> MDHNTFWFILIAFLFSGYFLLEGFDFGVGILAPIIGKDSAARNTVIRTIGPVWDGNEVWLIVAGGALFAAFPEWYATMFSGMYLPLFLVLVSLIIRVVGLEWRKKVDDPRWQKWSDRAIFIGSWTPPLMWGFIFANILRGMPIKADHTIDAAAALPGMVNVFAILGALAFTALFALHGLAFIRLKTAGRVRTDAAKAAPGVALLAAVTGGPFVLWAAIAYGRSWSWILAVLIIAAVLGGAFALIKDRDGLSFLSTSVAVIGVVALL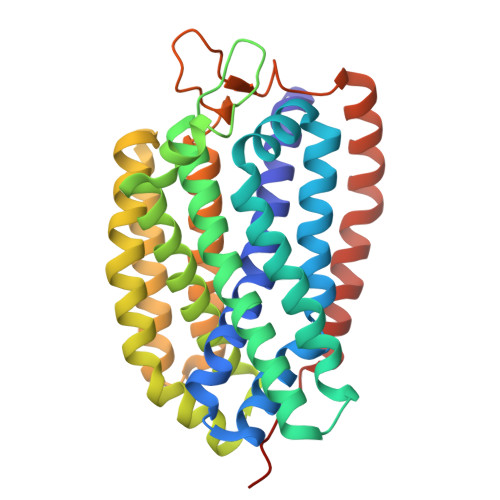FSSLFPNVMPTTLADGVSLDIWNASASHYALTILTWTAAVIAPLVVLYQGWTYWVFRKRLHAEPVSA> SSPPVVDTVHGKVLGKFVSL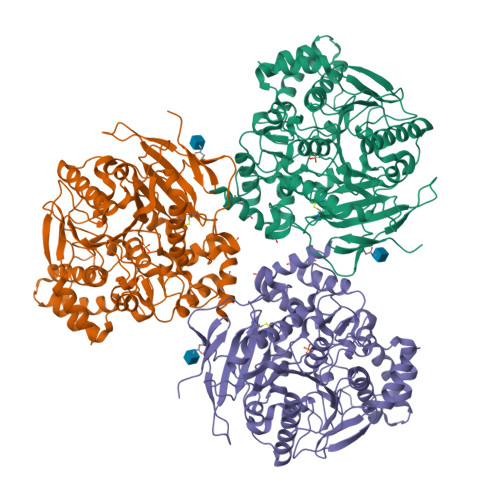EGFAQPVAIFLGIPFAKPPLGPLRFTPPQPAEPWSFVKNATSYPPMCTQDPKAGQLLSELFTNRKENIPLKLSEDCLYLNIYTPADLTKKNRLPVMVWIHGGGLMVGAASTYDGLALAAHENVVVVTIQYRLGIWGFFSTGDEHSRGNWGHLDQVAALRWVQDNIASFGGNPGSVTIFGESAGGESVSVLVLSPLAKNLFHRAISESGVALTSVLVKKGDVKPLAEQIAITAGCKTTTSAVMVHCLRQKTEEELLETTLKMKFLSLDLQGDPRESQPLLGTVIDGMLLLKTPEELQAERNFHTVPYMVGINKQEFGWLIPMLMSYPLSEGQLDQKTAMSLLWKSYPLVCIAKELIPEATEKYLGGTDDTVKKKDLFLDLIADVMFGVPSVIVARNHRDAGAPTYMYEFQYRPSFSSDMKPKTVIGDHGDELFSVFGAPFLKEGASEEEIRLSKMVMKFWANFARNGNPNGEGLPHWPEYNQKEGYLQIGANTQAAQKLKDKEVAFWTNLFAK>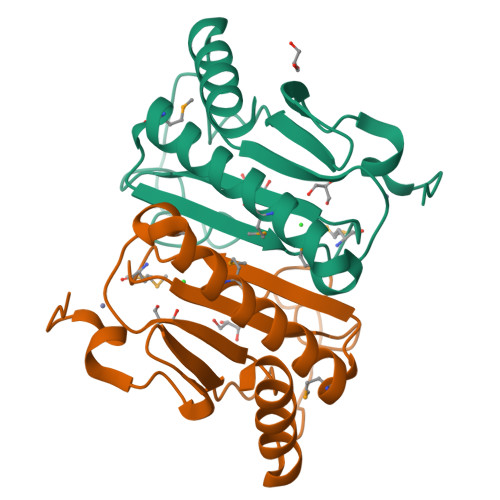GMTRTMSFHKNCELCTTAGGEILWQDALCRVVHVENQDYPGFCRVILNRHVKEMSDLRPAERDHLMLVVFAVEEAVREVMRPDKINLASLGNMTPHVHWHVIPRFKRDRHFPNSVWGETKRESLPQALDQGSTTALKKAISVRLDQGEPVFMGM[4x]>[2x]SACKETGWPFC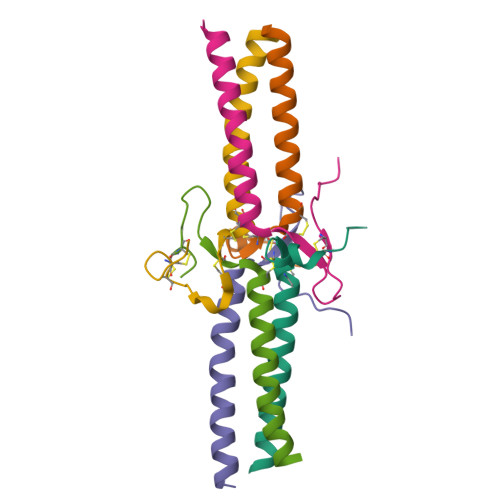SDEDWNTKCPSGCRMKGLIDEVDQDFTSRINKLRDSLFNYQK;>KVERKPPDADGCLHADPDLGVLCPTGCKLQDTLVRQERPIRKSIEDLRNTVDSVSR[2x];>[2x]YVATRDNCCILDERFGSYCPTTCGIADFLNNYQTSVDKDLRTLEGILY>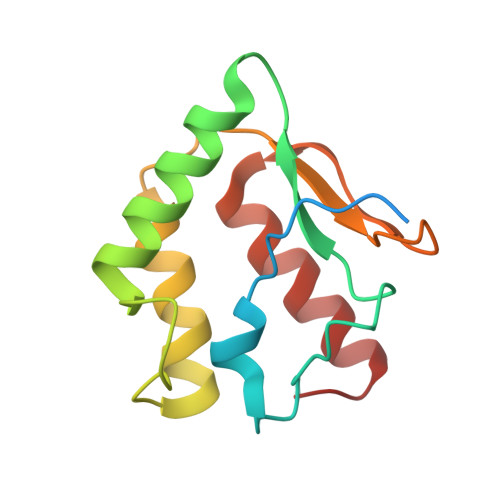 GSSHHHHHHENLYFQGMGVSESGHHVPAVRKSKGRPFEVSRFDKTRPTLFPRGENPEHSAWRLHHAERDVIGPRQGDFPGSDKELFDAYRKAYSKLDDIRVDVKSPNGTYTLGTNVTPSKAVDLIEVWLKGQGLM4'-HYDROXYMETHYL-4,5',8-TRIMETHYLPSORALEN | C15 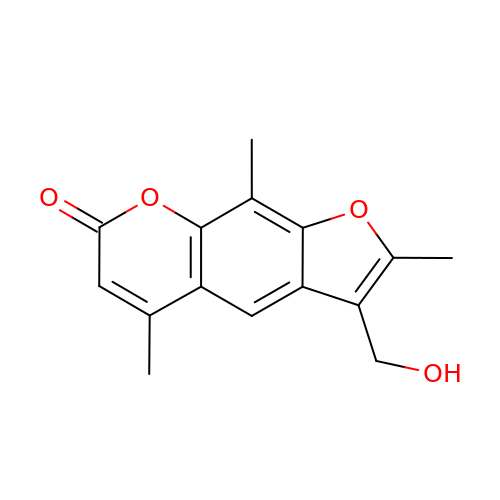H14 O4 | RGJSDHXSAKMPNM-UHFFFAOYSA-N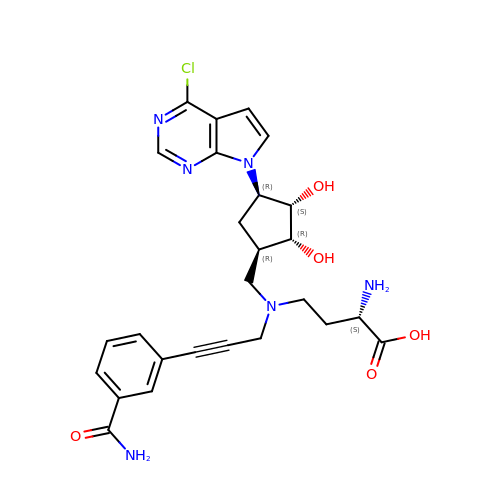(2S)-2-amino-4-([3-(3-carbamoylphenyl)prop-2-yn-1-yl]{[(1R,2R,3S,4R)-4-(4-chloro-7H-pyrrolo[2,3-d]pyrimidin-7-yl)-2,3-dihydroxycyclopentyl]methyl}amino)butanoic acid | C26 H29 Cl N6 O5 | JIYDUPLVTSNGNC-BLCKVISQSA-N>MVTTLTPVICESAPAAAASYSHAMKVNNLIFLSGQIPVTPDNKLVEGSIADKAEQVIQNIKNVLEA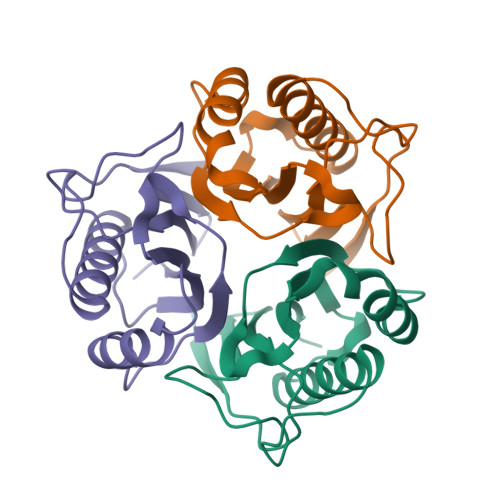SNSSLDRVVKVNIFLADINHFAEFNSVYAKYFNTHKPARSCVAVAALPLGVDMEMEAIAAERD[6x]>MGSSHHHHHHSSGLVPRGSHMASGLYPSYNTSPAAPDSTGMQSTAVQLAGKIRLGWNIGNTMEAIGGETAWGNPMVSNELLKLVKDSGFDAVRIPVAWDQYANQESAEISAAWLNRVKQVVQMAIDNELYVLINIHWDGGWLENNITPAKKDENNAKQKAFWEQIATHLRDFDEHLLFAGTNEPNAENAEQMDVLNSYLQTFVDAVRSTGGKNAYRVLVLQGPVTDIEKTNELWTHMPADTATDRLMAEVHFYTPYNFALMRQDESWGKQFYYWGEGFLSTTDTERNPTWGE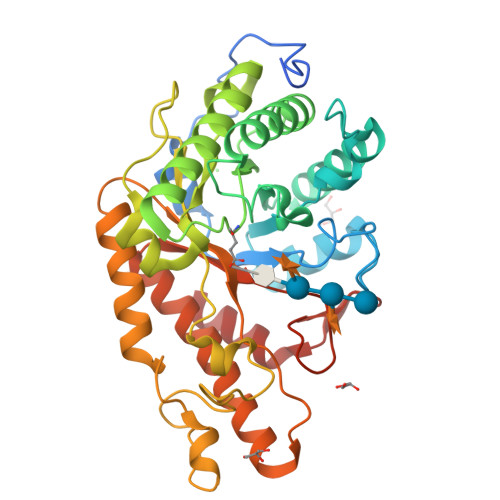EATIDQLFDLMKTKFVDQGIPVVLGEFSAMRRTNLTGDALTLHLAGRAYYHKYVTQQALARGLLPFYWDNGGNDNFSSGIFNRQQNTVFDQQVLDALLEGAGAQ[2x]> GPGSAVPFVEDWRLVQTLGEGAYGEVQL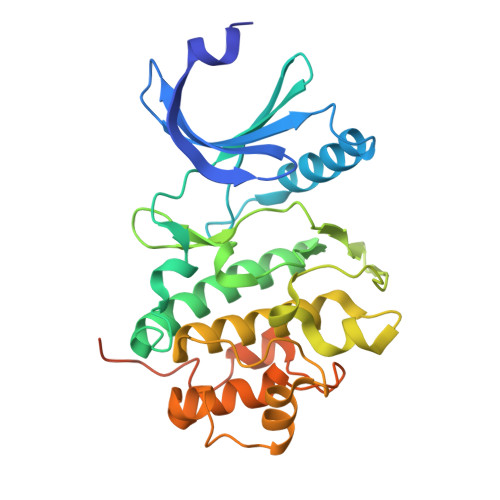AVNRVTEEAVAVKIVDMKRAVDCPENIKKEICINKMLNHENVVKFYGHRREGNIQYLFLEYCSGGELFDRIEPDIGMPEPDAQRFFHQLMAGVVYLHGIGITHRDIKPENLLLDERDNLKISDFGLATVFRYNNRERLLNKMCGTLPYVAPELLKRREFHAEPVDVWSCGIVLTAMLAGELPWDQPSDSCQEYSDWKEKKTYLNPWKKIDSAPLALLHKILVENPSARITIPDIKKDRWYNKPLKKGAKRPRVTSGGVSESPSGHHHHHHHH>[4x]ANEPIQPIKAVTPENADMAELGKMLFF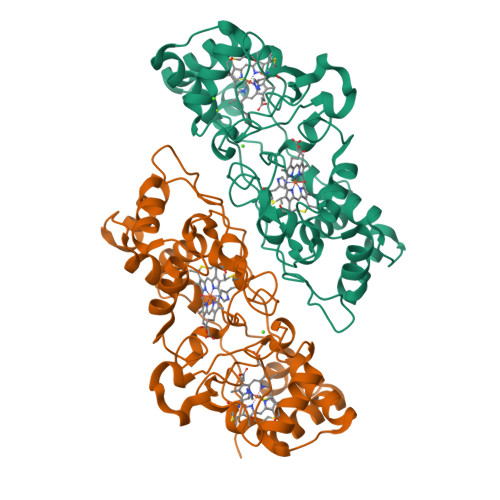DPRLSKSGFISCNSCHNLSMGGTDNITTSIGHKWQQGPINAPTVLNSSMNLAQFWDGRAKDLKEQAAGPIANPKEMASTHEIAEKVVASMPQYRERFKKVFGSDEVTIDRITTAIAQFEETLVTPGSKFDKWLEGDKNALNQDELEGYNLFKGSGCVQCHNGPAVGGSSYQKMGVFKPYETKNPAAGRMDVTGNEADRNVFKVPTLRNIELTYPYFHDGGAATLEQAVETMGRIQLNREFNKDEVSKIVAFLKTLTGDQPDFKLPILPPSNNDTPRSQPYE4-{5-(6-methoxynaphthalen-2-yl)-1-methyl-2-[2-methyl-4-(methylsulfonyl)phenyl]-1H-imidazol-4-yl}pyridine 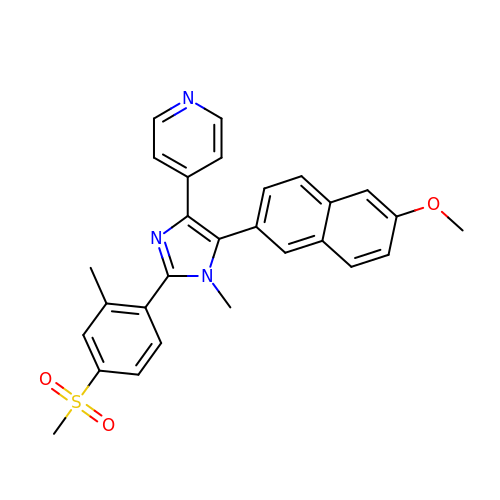| C28 H25 N3 O3 S | ZDSNJSQTPLXCSG-UHFFFAOYSA-N> MCWAAAIPIAISGAQAISGQNAQAKMIAAQTAAGRRQAMEIMRQTNIQNADLSLQ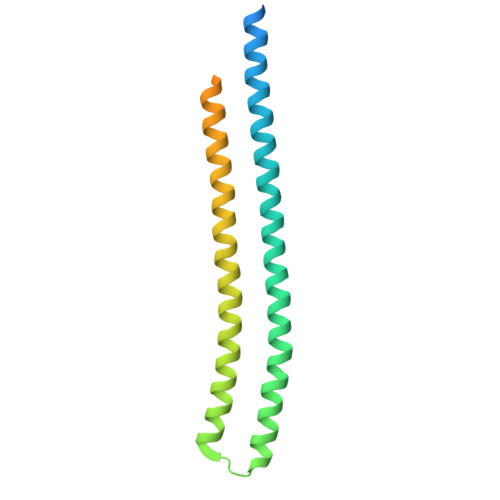ARSKLEEASAELTSQNMQKVQAIGSIRAAIGESMLEGSSMDRIKRVTEGQFIREANMVTENYRRDYQAIFAQQLGGTQSAASQIDEIYKSEQKQKSKLQMVLDPLAIMGSSAASAYASGAFDSKSTTKAPIVAAKGTKTGR> MGLLDRLSGLLGLKKKEVHVLCLGLDNSGKTTIINKLKPSNAQSQDIVPTIGFSIQKFKSSSLSFTVFDMSGQGRYRNLWEHYYKEGQAIIFVIDSSDKLRMVVAKEELRT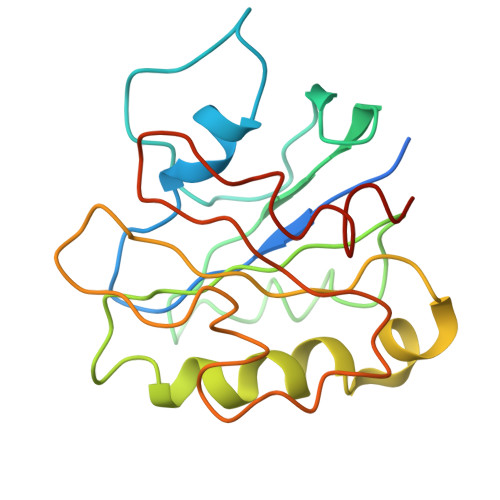LLNHPDIKHRRIPILFFANKMDLRDALTSVKVSQLLCLEDIKDKPWHICASDAIKGEGLQEGVDWLQDQIQSVKT> LKESPSGYLRSGEGDTGCGELVWVGEPLTLRTAETITGKYGVWMRDPKPTYPYTQETTWRIDTVGTDVRQVFEYDIISQFMQGYPSKVHILPRPLESTGAVVYSGSL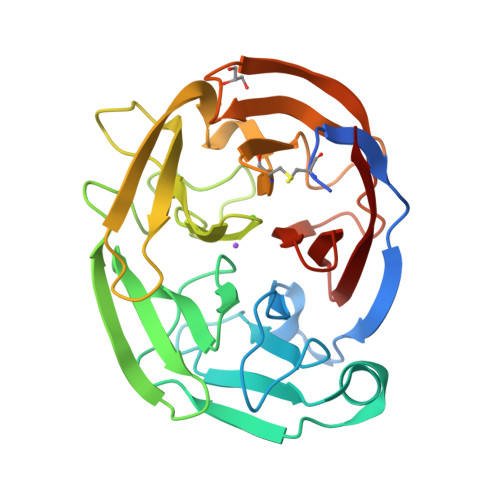YFQGAESRTVIRYELNTETVKAEKEIPGAGYHGQFPYSWGGYTDIDLAVDEAGLWVIYSTDEAKGAIVLSKLNPENLELEQTWETNIRKQSVANAFIICGTLYTVSSYTSADATVNFAYDTGTGISKTLTIPFKNRYKYSSMIDYNPLEKKLFAWDNLNMVTYDIKLSKM N-[(4S)-4,5-diamino-5-oxopentyl]-10-phenyldecanamide | C21 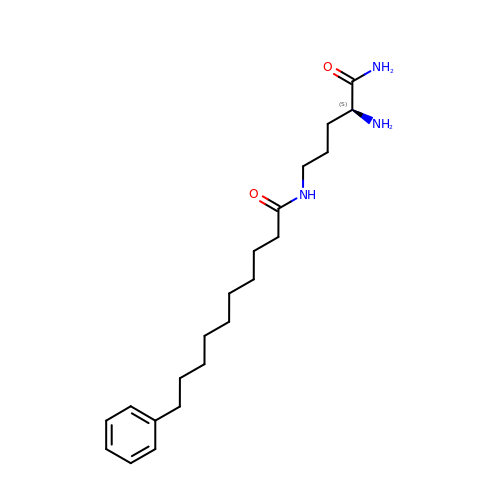H35 N3 O2 | PXLGZFSIHCIIGA-IBGZPJMESA-N>MNAYYIQDRLEAQSWARHYQQLAREEKEAELADDMEKGIPQHLFESLCIDHLQRHGASKKSITRAFDDDVEFQERMAEHIRYMVETIAHHQVDIDSEV[2x];> GMSDVAETLDPLRLPLQGERLIEASAGTGKTFTIAALYLRLLLGLGGSAAFPRPLTVEELLVVTFTEAATAELRGRIRSNIHELRIACLRETTDNPLYERLLEEIDDKAQAAQWLLLAERQMDEAAVFTIHGFCQRMLNLNAFESGMLFEQQLIEDESLLRYQACADFWRRHCYPLPREIAQVVFETWKGPQALLRDINRYLQGEAPVIKAPPPDDETLASRHAQIVARIDTVKQQWRDAVGELDALIESSGIDRRKFNRSNQAKWIDKISAWAEEETNSYQLPESLEKFSQRFLEDRTKAGGETPRHPLFEAIDQLLAEPLSIRDLVITRALAEIRETVAREKRRRGELGFDDMLSRLDSALRSESGEVLAAAIRTRFPVAMIDEFQDTDPQQYRIFRRIWHHQPETALLLIGDPKQAIYAFRGADIFTYMKARSEVHAHYTLDTNWRSAPGMVNSVNKLFSQTDDAFMFREIPFIPVKSAGKNQALRFVFKGETQPAMKMWLMEGESCGVGDYQSTMAQVCAAQIRDWLQAGQRGEALLMNGDDARPVRASDISVLVRSRQEAAQVRDALTLLEIPSVYLSNRDSVFETLEAQEMLWLLQAVMTPERENTLRSALATSMMGLNALDIETLNNDEHAWDVVVEEFDGYRQIWRKRGVMPMLRALMSARNIAENLLATAGGERRLTDILHISELLQEAGTQLESEHALVRWLSQHILEPDSNASSQQMRLESDKHLVQIVTIHKSKGLEYPLVWLPFITNFRVQEQAFYHDRHSFEAVLDLNAAPESVDLAEAERLAEDLRLLYVALTRSVWHCSLGVAPLVRRRGDKKGDTDVHQSALGRLLQKGEPQDAAGLRTCIEALCDDDIAWQTAQTGDNQPWQVNDVSTAELNAKTLQRLPGDNWRVTSYSGLQQRGHGIAQDLMPRLDVDAAGVASVVEEPTLTPHQFPRGASPGTFLHSLFEDLDFTQPVDPNWVREKLELGGFESQWEPVLTEWITAVLQAPLNETGVSLSQLSARNKQVEMEFYLPISEPLIASQLDTLIRQFDPLSAGCPPLEFMQVRGMLKGFIDLVFRHEGRYYLLDYKSNWLGEDSSAYTQQAMAAAMQAHRYDLQYQLYTLALHRYLRHRIADYDYEHHFGGVIYLFLRGVDKEHPQQGIYTTRPNAGLIALMDEMFAGMTLEEA;> MLRVYHSNRLDVLEALMEFIVERERLDDPFEPEMILVQSTGMAQWLQMTLSQKFGIAANIDFPLPASFIWDMFVRVLPEIPKESAFNKQSMSWKLMTLLPQLLEREDFTLLRHYLTDDSDKRKLFQLSSKAADLFDQYLVYRPDWLAQWETGHLVEGLGEAQAWQAPLWKALVEYTHQLGQPRWHRANLYQRFIETLESATTCPPGLPSRVFICGISALPPVYLQALQALGKHIEIHLLFTNPCRYYWGDIKDPAYLAKLLTRQRRHSFEDRELPLFRDSENAGQLFNSDGEQDVGNPLLASWGKLGRDYIYLLSDLESSQELDAFVDVTPDNLLHNIQSDILELENRAVAGVNIEEFSRSDNKRPLDPLDSSITFHVCHSPQREVEVLHDRLLAMLEEDPTLTPRDIIVMVADIDSYSPFIQAVFGSAPADRYLPYAISDRRARQSHPVLEAFISLLSLPDSRFVSEDVLALLDVPVLAARFDITEEGLRYLRQWVNESGIRWGIDDDNVRELELPATGQHTWRFGLTRMLLGYAMESAQGEWQSVLPYDESSGLIAELVGHLASLLMQLNIWRRGLAQERPLEEWLPVCRDMLNAFFLPDAETEAAMTLIEQQWQAIIAEGLGAQYGDAVPLSLLRDELAQRLDQERISQRFLAGPVNICTLMPMRSIPFKVVCLLGMNDGVYPRQLAPLGFDLMSQKPKRGDRSRRDDDRYLFLEALISAQQKLYISYIGRSIQDNSERFPSVLVQELIDYIGQSHYLPGDEALNCDESEARVKAHLTCLHTRMPFDPQNYQPGERQSYAREWLPAASQAGKAHSEFVQPLPFTLPETVPLETLQRFWAHPVRAFFQMRLQVNFRTEDSEIPDTEPFILEGLSRYQINQQLLNALVEQDDAERLFRRFRAAGDLPYGAFGEIFWETQCQEMQQLADRVIACRQPGQSMEIDLACNGVQITGWLPQVQPDGLLRWRPSLLSVAQGMQLWLEHLVYCASGGNGESRLFLRKDGEWRFPPLAAEQALHYLSQLIEGYREGMSAPLLVLPESGGAWLKTCYDAQNDAMLDDDSTLQKARTKFLQAYEGNMMVRGEGDDIWYQRLWRQLTPETMEAIVEQSQRFLLPLFRFNQS;> MGKLQKQLLEAVEHKQLRPLDVQFALTVAGDEHPAVTLAAALLSHD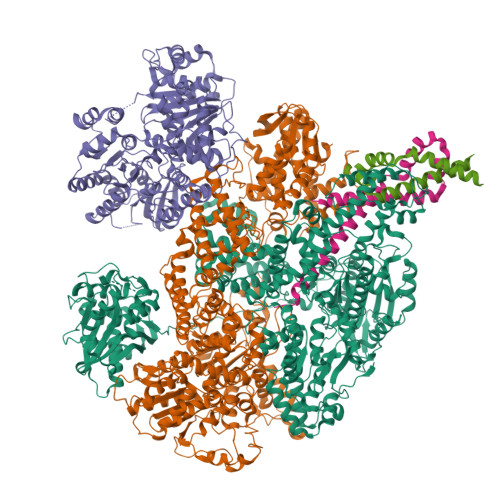AGEGHVCLPLSRLENNEASHPLLATCVSEIGELQNWEECLLASQAVSRGDEPTPMILCGDRLYLNRMWCNERTVARFFNEVNHAIEVDEALLAQTLDKLFPVSDEINWQKVAAAVALTRRISVISGGPGTGKTTTVAKLLAALIQMADGERCRIRLAAPTGKAAARLTESLGKALRQLPLTDEQKKRIPEDASTLHRLLGAQPGSQRLRHHAGNPLHLDVLVVDEASMIDLPMMSRLIDALPDHARVIFLGDRDQLASVEAGAVLGDICAYANAGFTAERARQLSRLTGTHVPAGTGTEAASLRDSLCLLQKSYRFGSDSGIGQLAAAINRGDKTAVKTVFQQDFTDIEKRLLQSGEDYIAMLEEALAGYGRYLDLLQARAEPDLIIQAFNEYQLLCALREGPFGVAGLNERIEQFMQQKRKIHRHPHSRWYEGRPVMIARNDSALGLFNGDIGIALDRGQGTRVWFAMPDGNIKSVQPSRLPEHETTWAMTVHKSQGSEFDHAALILPSQRTPVVTRELVYTAVTRARRRLSLYADERILSAAIATRTERRSGLAALFSSRE> GSMASAAQLRIQKDINELNLPKTCDISFSDPDDLLNFKLVICPDEGFYKSGKFVFSFKVGQGYPHDPPKVKCETMVYHPNIDLEGNVCLNILREDWKPVLTINSIIYGLQYLFLEPNPEDPLNKEAAEVLQNNRRLFEQNVQRSMRGGYIGSTYFERCLK;> GSSQLPQNIQFSPSAKLQEVLDYLTNSA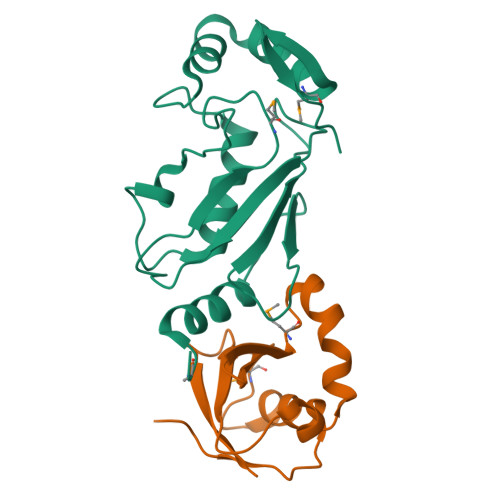SLQMKSPAITATLEGKNRTLYMQSVTSIEERTRPNLSKTLKELGLVDGQELAVADVTTPQTVLFKLHFTS> MIEIKDKQLTGLRFIDLFAGLGGFRLALESCGAECVYSNEWDKYAQEVYEMNFGEKPEGDITQVNEKTIPDHDILCAGFPCQAFSISGKQKGFEDSRGTLFFDIARIVREKKPKVVFMENVKNFASHDNGNTLEVVKNTMNELDYSFHAKVLNALDYGIPQKRENIYMICFRNDLNIQNFQFPKPFELNTFVKDLLLPDSEVEHLVID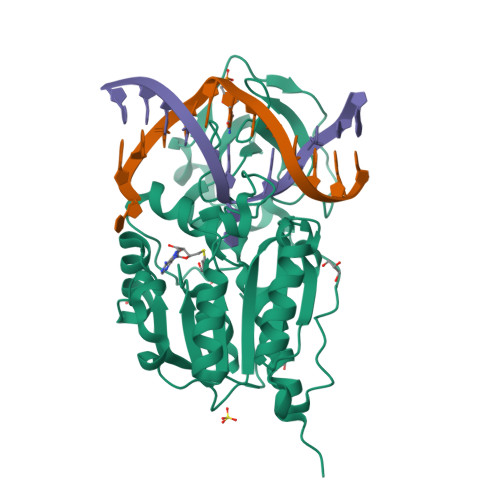RKDLVMTNQEIEQTTPKTVRLGIVGKGGQGERIYSTRGIAITLSAYGGGIFAKTGGYLVNGKTRKLHPRECARVMGYPDSYKVHPSTSQAYKQFGNSVVINVLQYIAYNIGSSLNFKPY> MKLERVTVKNFRSHSDTVVEFKEGINLIIGQNGSGKSSLLDAILVGLYWPLRIKDIKKDEFTKVGARDTYIDLIFEKDGTKYRITRRFLKGYSSGEIHAMKRLVGNEWKHVTEPSSKAISAFMEKLIPYNIFLNAIYIRQGQIDAILES;> KYKALAREAALSKIGELASEIFAEFTEG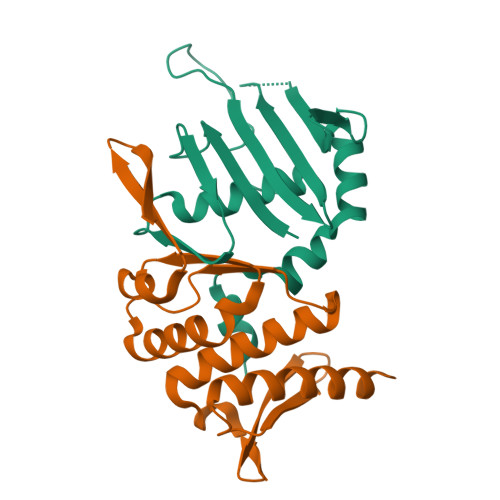KYSEVVVRAEENKVRLFVVWEGKERPLTFLSGGERIALGLAFRLAMSLYLAGEISLLILDEPTPYLDEERRRKLITIMERYLKKIPQVILVSHDEELKDAADHVIRISLENGSSKVEVVS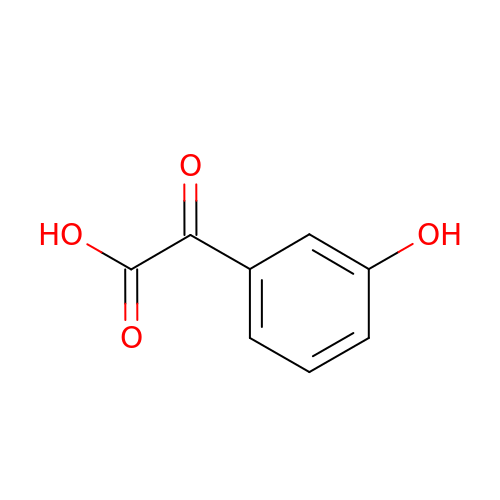2-(3-HYDROXYPHENYL)-2-OXO-ETHANOIC ACID | C8 H6 O4 | NBDYDHVCTKPDRI-UHFFFAOYSA-N>QTEQGANISDQWTGSELPLAFASDSNPSDPVSNVNDKLISYNNQPANRWTNWNRSNPEASVGVLFGDSGILSKRSVDNLSVGFHEDHGVGAPKSYVIEYYVGKTVPTAPKNPSFVGNEDHVFNDSANWKPVTNLKAPAQLKAGEMNHFSFDKVETYAIRIRMVKADNKRGTSITEVQIFAKQV[2x]

BgaA is specific for galactose β-1,4-linked to glucose or GlcNAc [lactose or N-acetyllactosamine (LacNAc) motifs, respectively] found in glycoconjugates. The N-terminal region of BgaA comprising amino acid residues 138–993 has amino acid sequence identity with GH family 2 enzymes. Through detailed structural and functional analyses the molecular basis for the catalytic specificity of BgaA is defined and this activity is demonstrated as critical for the ability of pneumococci to utilize complex N-linked glycans as a carbon source and protect the bacterium from opsonophagocytic killing. Further analyses also revealed the presence of non-catalytic CBMs within the C-terminal region of BgaA that mediate adherence to host cell surface LacNAc and/or lactose.

However, fold prediction using the Phyre2 server, which does not rely on amino acid sequence similarity, distinguished two regions (XII and XV) with a high probability of adopting the β-sandwich fold common to many CBMs found in CAZymes. The two predicted CBMs were recombinantly produced and the polypeptides screened for binding to all commonly occurring monosaccharides by UV difference spectroscopy; only D-galactose gave a signature UV difference spectrum consistent with sugar binding. Subsequently, this approach was expanded to the relevant galactose-containing sugars LacNAc, lactose, galactopyranosyl-β-1,3-N-acetyl-D-glucosamine (lacto-N-biose), and galactopyranosyl-β-1,3-N-acetyl-D-galactosamine [Thomsen-Freidenreich (TF) epitope] and binding was only observed to LacNAc and lactose. Significantly, the CBMs only bound with significant affinity to sugars that are substrates for the catalytic domain. A single bound metal ion was modeled as Ca2+ on the basis of coordination geometry and B-factor analysis. The shallow LacNAc binding site sits at the apex of the β-fold opposite the N- and C-termini. Tryptophan 1514 lies directly beneath the glycoside bond and coplanar with the disaccharide thus providing CH-π interactions with both pyranose rings and a higher affinity for β-linked disaccharides than for galactose alone. This binding site architecture accommodates lactose and LacNAc, but would limit the recognition of other sugars terminating in β-linked galactose.Kalimantacin | C30 H48 N2 O7 | 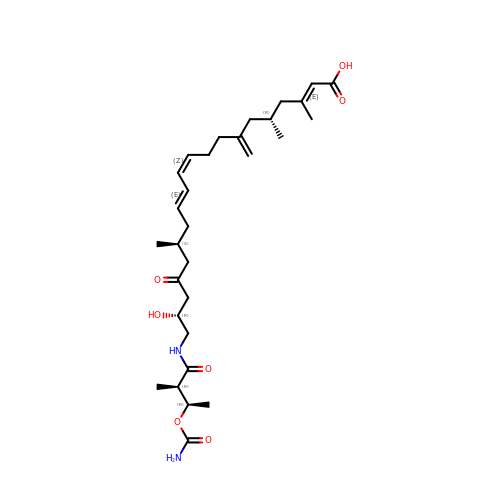GENAAYFYLGYPIQ-DPTWSAQQSA-N> QDFPTRPLSRFIP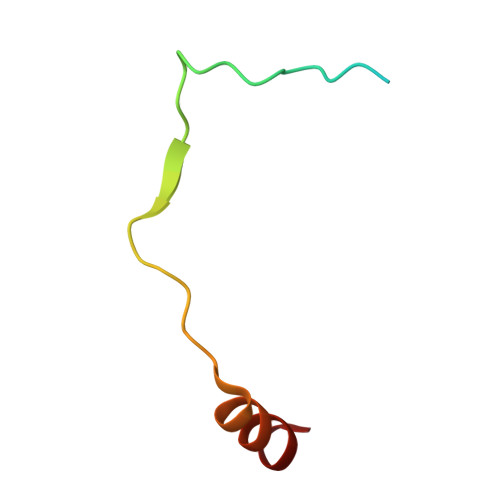WFPYDGSKLPLRPKRSPPVISEEAAEDVKQYLT All Shewanella capable of EET contain an mtr gene cluster that encodes for MtrCAB, a porin‐cytochrome complex that transports electrons across the outer membrane and reduces extracellular electron acceptors (Fredrickson et al., 2008). An outer membrane cytochrome (OMC) termed MtrC binds to the surface of MtrAB and can directly transfer electrons to extracellular terminal acceptors (Edwards et al., 2020; White et al., 2013). Shewanella oneidensis MtrC is composed of four domains, with the hemes closely packed and distributed evenly between domains II and IV. In both MtrC and OmcA, the first five hemes are located within domain II, and hemes 6–10 are within domain IV.

Site‐directed mutagenesis allowed the production of a truncated MtrC variant comprised solely of domains I and II (MtrCDI,II) that is near‐identical to domains I and II of the full‐length MtrC. Upon sample reduction, there was a shift in the Soret peak maximum from 410 to 420 nm and a sharpening of the α and β bands (maxima at 552 and 525 nm, respectively). These spectral features are typical of redox‐active, low‐spin, bis‐histidine coordinated c‐type hemes, and together with the LC–MS, indicate the protein consists of a soluble MtrC pentaheme cytochrome mainly truncated at amino acid residue 325. X‐ray crystallography was used to determine the molecular structure of MtrCDI,II,sol to a resolution of 1.8 Å. The structure confirmed the successful assembly of MtrCDI,II,sol, including the covalent attachment of five bis‐histidine coordinated c‐type hemes. The orientation of the 10 histidine imidazole rings that form the axial ligands to the heme irons is also highly conserved (RMSD of 0.225 Å), suggesting that the environment of the five hemes was unchanged. The redox potential window of MtrCDI,II,sol was similar to the observed window for MtrCsol measured under comparable conditions. Thus, there is no evidence that either the N‐ or the C‐terminal domain of the full‐length protein holds the majority of hemes with the more negative reduction potentials. The biophysical, structural, and spectroscopic evidence showed that the MtrCDI,II,sol pentaheme cytochrome was structurally homologous to the equivalent domains of MtrC. In our experiments, the addition of a stop codon to mtrC resulted in the assembly of a truncated MtrCDI,II variant, with domains I and II both structurally and spectroscopically identical to the corresponding domains of the full‐length protein. This MtrCDI,II could interact with MtrAB, resulting in the formation of a 15‐heme MtrCDI,IIAB nanowire capable of reducing a limited number of substrates, but unable to reduce the key physiological substrates FMN and Fe(III) citrate. The in vivo catalytic experiments presented here demonstrate that the reduction of physiological substrates requires the full 4‐domain structure of MtrC, yet reduction of certain other substrates is still achievable via the 2‐domain MtrC.

> MKFKLNLITLALLANTGLAVAADGGSDGNNGNDGSDGGEPAGSIQTLNLDITKVSYENGAPMVTVFATNEADMPVIGLANLEIKKALQLIPEGATGPGNSANWQGLGSSKSYVDNKNGSYTFKFDAFDSNKVFNAQLTQRFNVVSAAGKLADGTTVPVAEMVEDFDGQGNAPQYTKNIVSHEVCASCHVEGEKIYHQATEVETCISCHTQEFADGRGKPHVAFSHLIHNVHNANKAWGKDNKIPTVAQNIVQDNCQVCHVESDMLTEAKNWSRIPTMEVCSSCHVDIDFAAGKGHSQQLDNSNCIACHNSDWTAELHTAKTTA> XSAWSH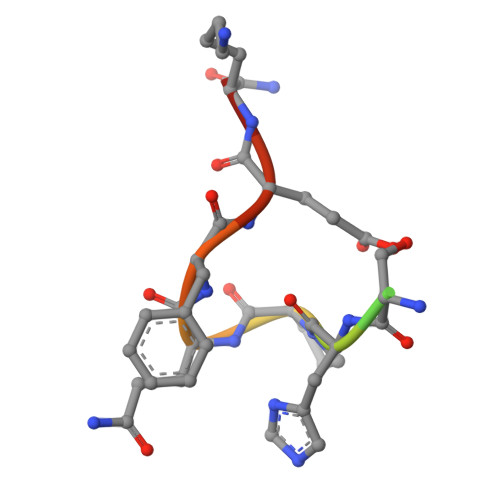PQFEKX> GIKKPV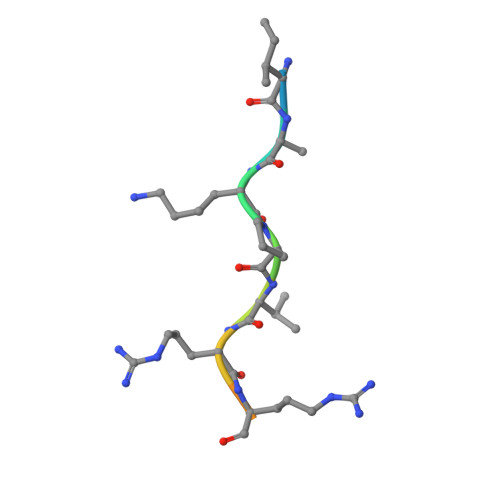RRKLKE>[2x]GSHMNGSIQGKPLLGKGMSESLTGTLDAPFPEYQTLPADPMSVLHNWLERARRVGIREPRALALATADSQGRPSTRIVVISEISDAGVVFST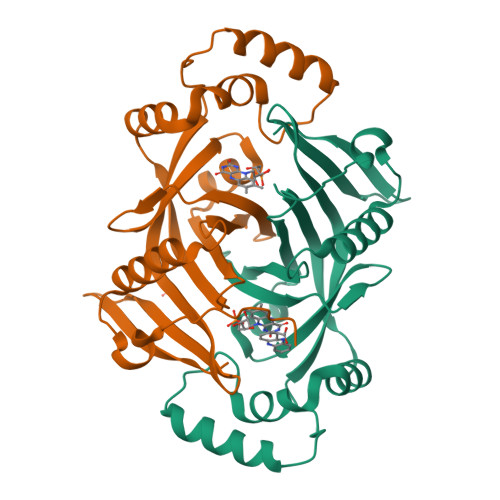HAGSQKGRELLHNPWASGVLYWRETSQQIILNGQAVRLPNAKADDAWLKRPYATHPMSSVSRQSEELQDVQAMRNAARQLAELQGPLPRPEGYCVFELRLESLEFWGNGQERLHERLRYDRSDTGWNVRRLQP> MNIPKPADSTWTDDQWNAIVSTGQDILVAAAAGSGKTAVLVERMIRKITAEENPIDVDRLLVVTFTNASAAEMKHRIAEALEKELVQRPGSLHIRRQLSLLNRASISTLHSFCLQVLKKYYYLIDLDPGFRIADQTEGELIGDEVLDELFEDEYAKGEKAFFELVDRYTTDRHDLDLQFLVKQVYEYSRSHPNPEAWLESFVHLYDVSEKSAIEELPFYQYVKEDIAMVLNGAKEKLLRALELTKAPGGPAPRADNFLDDLAQIDELIQHQDDFSELYKRVPAVSFKRAKAVKGDEFDPALLDEATDLRNGAKKLLEKLKTDYFTRSPEQHLKSLAEMKPVIETLVQLVISYGKRFEAAKQEKSIIDFSDLEHYCLAILTAENDKGEREPSEAARFYQEQFHEVLVDEYQDTNLVQESILQLVTSGPEETGNLFMVGDVKQSIYRFRLAEPLLFLSKYKRFTESGEGTGRKIDLNKNFRSRADILDSTNFLFKQLMGGKIGEVDYDEQAELKLGAAYPDNDETETELLLIDNAEDTDASEEAEELETVQFEAKAIAKEIRKLISSPFKVYDGKKKTHRNIQYRDIVILLRSMPWAPQIMEELRAQGIPVYANLTSGYFEAVEVAVALSVLKVIDNPYQDIPLASVLRSPIVGADEN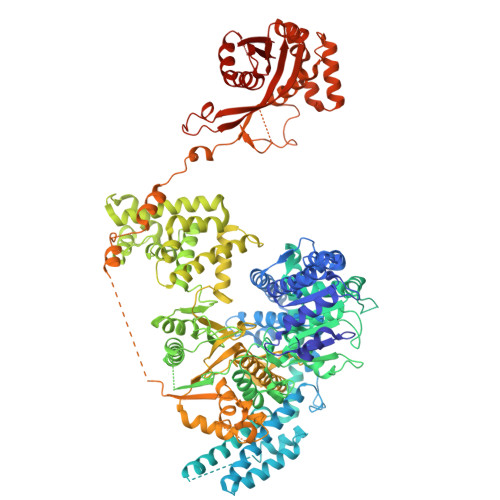ELSLIRLENKKAPYYEAMKDYLAAGDRSDELYQKLNTFYGHLQKWRAFSKNHSVSELIWEVYRDTKYMDYVGGMPGGKQRQANLRVLYDRARQYESTAFRGLFRFLRFIERMQERGDDLGTARGLSEQEDVVRLMTIHSSKGLEFPVVFVAGLGRNFNMMDLNKSYLLDKELGFGTKYIHPQLRISYPTLPLIAMKKKMRRELLSEELRVLYVALTRAKEKLFLIGSCKDHQKQLAKWQASASQTDWLLPEFDRYQARTYLDFIGPALARHRDLGDLAGVPAHADISGHPARFAVQMIHSYDLLDDDLEERMEEKSERLEAIRRGEPVPGSFAFDEKAREQLSWTYPHQEVTQIRTKQSVSEIKRKREYEDEYSGRAPVKPADGSILYRRPAFMMKKGLTAAEKGTAMHTVMQHIPLSHVPSIEEAEQTVHRLYEKELLTEEQKDAIDIEEIVQFFHTEIGGQLIGAKWKDREIPFSLALPAKEIYPDAHEADEPLLVQGIIDCLYETEDGLYLLAYKSDRIEGKFQHGFEGAAPILKKRYETQIQLYTKAVEQIAKTKVKGCALYFFDGGHILTL>LHLDQTPSRQPIPSEGLQLHLPQVLADAVSRLVLGKFGDLTDNFSSPHARRKVLAGVVMTTGTDVKDAKVISVSTGTKCINGEYMSDRGLALNDCHAEIISRRSLLRFLYTQLELYLNNKDDQKRSIFQKSERGGFRLKENVQFHLYISTSPCGDARIFSPHEPILEEPADRHPNRKARGQLRTKIESGYGTIPVRSNASIQTWDGVLQGERLLTMSCSDKIARWNVVGIQGSLLSIFVEPIYFSSIILGSLYHGDHLSRAMYQRISNIEDLPPLYTLNKPLLSGISNAEARQPGKAPNFSVNWTVGDSAIEVINATTGKDELGRASRLCKHALYCRWMRVHGKVPSHLLRSKITKPNVYHESKLAAKEYQAAKARLFTAFIKAG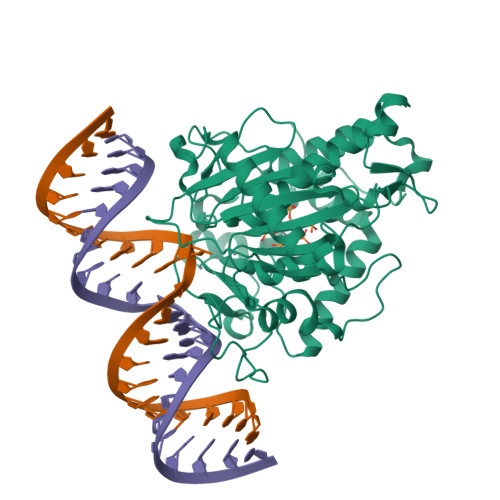LGAWVEKPTEQDQFSLTP[2x]>MRGSFVEMVDNLRGKSGQGYYVEMTVGSPPQTLNILVDTGSSNFAVGAAPHPFLHRYYQRQLSSTYRDLRKGVYVPYTQGKWEGELGTDLVSIPHGPNVTVRANIAAITESDKFFINGSNWEGILGLAYAEIARPDDSLEPFFDSLVKQTHVPNLFSLQLCGAGFPLNQSEVLASVGGSMIIGGIDHSLYTGSLWYTPIRREWYYEVIIVRVEINGQDLKMDCKEYNYDKSIVDSGTTNLRLPKKVFEAAVKSIKAASSTEKFPDGFWLGEQ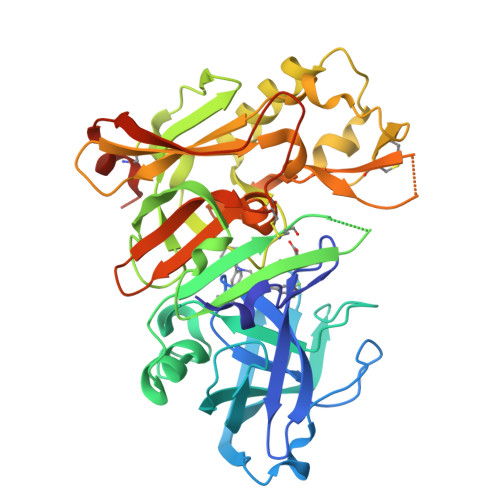LVCWQAGTTPWNIFPVISLYLMGEVTNQSFRITILPQQYLRPVEDVATSQDDCYKFAISQSSTGTVMGAVIMEGFYVVFDRARKRIGFAVSACHVHDEFRTAAVEGPFVTLDMEDCGYNIPQTDESRSHHHHHH[3x]6-deoxy-2,3-di-O-methyl-alpha-L-mannopyranose | C8 H16 O5 | 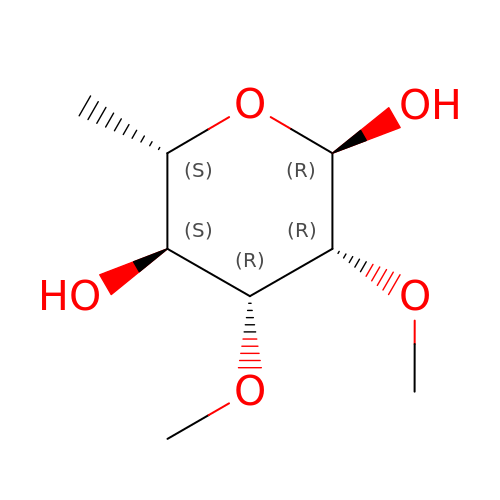SXWBIRCAXZNEGK-TVNFTVLESA-N> MLPNTKLHNTIFSETRKFTRESFKEIEHLTARLAND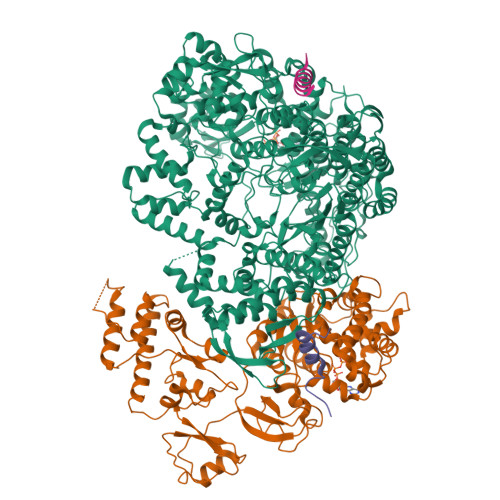RVARHDFLFNTSIVLISDYSGEDSNGNQLQATITIPNEIINPKEYDPSDYPLAEDESFFKQGHKYDYLVTFRAGSLTNTYEPKTKMYKLHAALDKLMHVKQRKSRFADLWRELCAVIASLDVWYQTTNYPLRTYVKLLFHKGDEFPFYESPSQDRIIFNDKSVASILPTFVYTCCQVGTAIMSGILTHVESIVAMNHFLHCAKDSYIDEKLKIKGIGRSWYQEALHNVCQATVPVWSQFNEVIGHRTKSTSEPHFVSSTFISLRAKRAELLYPEFNAYINRAIQLSKTQNDVANYYAACRAMTNDGTFLATLTELSLDAAVFPRIEQHLVTRPAVLMSNTRHESLKQKYTNGVGSIAQSYLSSFTDEIAKRVNGRHHDEAWLNFLTTSSPGRKLTEIEKLEVGGDVAAWSNSRIVMQAVFAREYRTPERIFKSLKAPIKLVERQQSDRRQRAISGLDNDRLFLSFMPYTIGKQIYELNDNAAQGKQAGNAFDIGEMLYWTSQRNVLLSSIDVAGMDASVTTNTKDIYNTFVLDVASKCTVPRFGPYYAKNMEVFEAGNRQSQVRYVNAAWQACALEAANSQTSTSYESEIFGQVKNAEGTYPSGRADTSTHHTVLLQGLVRGNELKRASDGKNSCLATIKILGDDIMEIFQGSESDTYDHAVSNASILNESGFATTAELSQNSIVLLQQLVVNGTFWGFADRISLWTREDTKDIGRLNLAMMELNALIDDLVFRVRRPEGLKMLGFFCGAICLRRFTLSVDNKLYDSTYNNLSKYMTLTKYDKNPDSDSTLMSLILPLAWLFMPRGGEYPAYPFERRDGTFTEDESMFTARGAYKRRLLYDVSNIGEMIQQNSMALDDDLLHEYGFTGALLLIDLNILDLIDEVKKEDISPVKVSELATSLEQLGKLGEREKSRRAASDLKIRGHALSNDIVYGYGLQEKIQKSAMATKETTVQSKRVSSRLHDVIVAKTRDYKISTIPADALHLHEFEVEDVTVDLLPHAKHTSYSSLAYNMSFGSDGWFAFALLGGLDRSANLLRLDVASIRGNYHKFSYDDPVFKQGYKIYKSDATLLNDFFTAISAGPKEQGILLRAFAYYSLYGNVEYHYVLSPRQLFFLSDNPVSAERLVRIPPKYYVSTQCRALYNIFSYLHILRSIANNRGKRLKMVLHPGLIAYVRGTSQGAILPEADNV;> MFAIDPLKHSKLYEEYGLYLRPHQINQEIKPTTIKKKELAPTIRSIKYASLIHSMLAKHAARHNGTLINPRMYADMITLGNTKVTVTKGTPKAQIDTLKMNGLTVVSKSRRNNKKKPVSDTTATIDENTDDIVTYKALTEMSTLIESFRLPSGLALIIFDDEKYQSLIPNYINQLIAYTQPHIIPTWQGIADFSDTYLRSYFKRPFELTASNLAAPQKYNLSPMTRSIFNNTGREDAVIRKLYGYGEYVFIRYEGCLITWTGIYGEVTMMVNLSKRDLGLDVGDDYLKEYKKLLFYGVITDAIPSGISARSTIMKISPHKMMNPSGGALAVLSKFLEAVVSTNVINATLVVYAEKGAGKTSFLSTYAEQLSLASGQVVGHLSSDAYGRWLAKNKDVEEPSFAYDYVLSLDTDDNESYYEQKASELLISHGISEVAQYELLSVRKKIKMMDEMNEVLIAQLENADTHSERNFYYMVSTGKTTPRTLIVEGHFNAQDATIARTDTTVLLRTINDTTQAMRDRQRGGVVQLFLRDTYYRLLPALHTTVYPFEMLESIRRWKWVH;>[2x]PTVVQSRTDVFNEQFANEALHPMT> MGQNTLKVHDLNEDAEFDENGVEVFDEKALVEEEPSDNDLAEEELLSQGATQRVLDATQLYLGEIGYSPLLTAEEEVYFARRALRGDVASRRRMIESNLRLVVKIARRYGNRGLALLDLIEEGNLGLIRAVEKFDPERGFRFSTYATWWIRQTIERAIMNQTRTIRLPIHI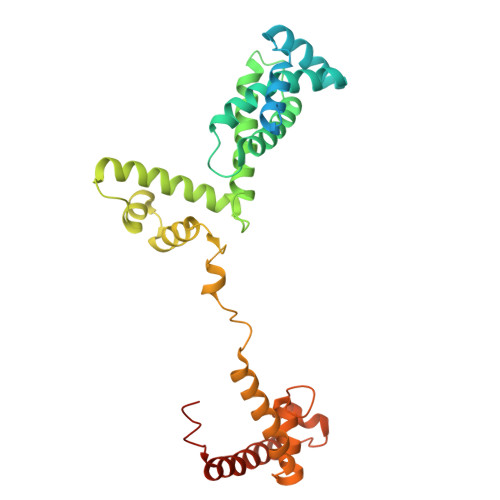VKELNVYLRTARELSHKLDHEPSAEEIAEQLDKPVDDVSRMLRLNERGTAVDTPLGGDSEKALLDILADEKENGPEDTTQDDDMKQSIVKWLFELNAKQREVLARRFGLLGYEAATLEDVGREIGLTRERVRQIQVEGLRRLREILQTQGLNIEALFLEHHHHHH>[4x]TTSAVNIYNISAGASVDLAAPVTTGDIVTFFSSALNLSAGAGSPNNTALNLLSENGAYLLHIAFRLQENVIVFNSRQPNAPWLV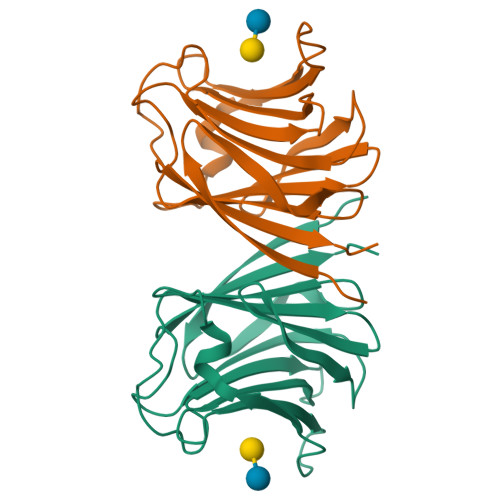EQRVSNVANQFIGSGGKAMVTVFDHGDKYQVVINEKTVIQYTKQISGTTSSLSYNSTEGTSIFSTVVEAVTYTGLA>MSSFVVPSLTAVRPRDHHDYADRIALSAATTDGVQMRTEDVRAWIAERRDANVFHVERIPFADLDQWWFEGVTGNLVHRSGRFFTIEGLHVIEHDGPHGDGPYREWQQPVIRQPEVGILGILAKEFDGVLHFLMQAKMEPGNPNLVQLSPTVQATRSNYTKAHGGTNVKLIEYFAPPDPERVIVDVLQAEQGSWFFRKSNRNMIVETVDDVPLWDDFCWLTLGQIAELMHEDETINMNSRSVLSCLPYQDITPRALFSDVQLLSWFTNERSRHDVRVRRIPLADVCGWKQGAEEIE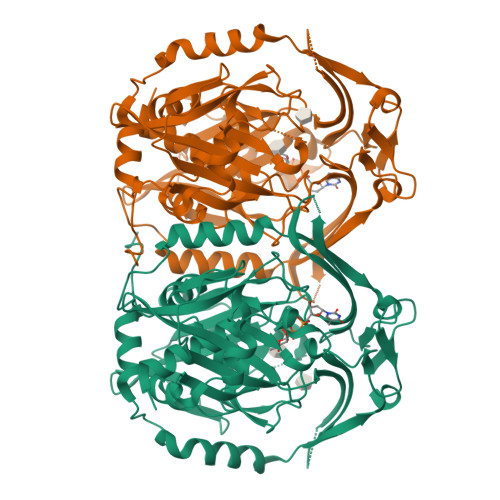HEDGRYFKVLAVAVKGSNREKISWTQPLVESVDLGVVAFLVRKIDGVPHVLVQARVDGGFLDTVELAPTVQCTPLNYAHLPAEEAPPFLDLVQNAPRSRIRYEAIHSEEGGRFLGVRARYLVIDADEAIDPPPGYAWVTPAQLTALTRHGHYVNVEARTLLACINAAAAQPRGGA[2x]>MHHHHHHSGRSVANQANLIDNKRELEQHALVPYAQGKSIHQLFEEQAEAFPDRVAIVFENRRLSYQELNRKANQLARALLEKGVQTDSIVGVMMEKSIENVIAILAVLKAGGAYVPIDIEYPRDRIQYILQDSQTKIVLTQKSVSQLVHDVGYSGEVVVLDEEQLDARETANLHQPSKPTDLAYVIYTSGTTGKPKGTMLEHKGIANLQSFFQNSFGVTEQDRIGLFASMSFDVSVSEMFMALLSGASLYILSKQTIHDFAAFEHYLSENELTIITLPPTYLTHLTPERITSLRIMITAGSASSAPLVNKWKDKLRYINAYGPTECLVATIWEAPSNQLSVQSVPIGKPIQNTHIYIVNEDLQLLPTGSEGELCIGGVGLARGYWNRPDLTAEKFVDNPFVPGE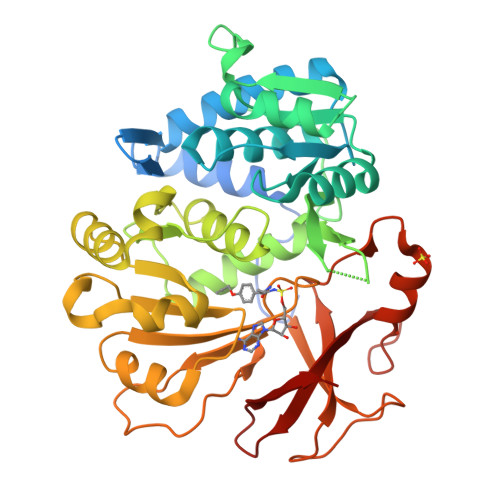KMYRTGDLAKWLTDGTIEFLGRI[2x]> MLPQDDMTDEMKSLASRLEDTTQA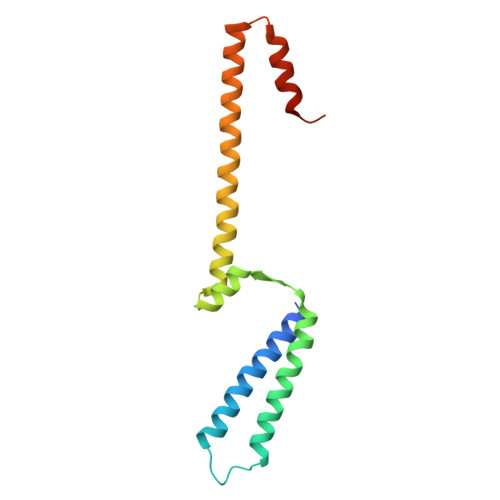FYDLALIVYNLEDTTPSDAIPESLDTLIRDLKSLPDISRKVNNLIPQDVLEYIEQGRNPDVYARQFSELVQKDNQYVNGKLYAIEGFQKAFAEEIKQAYPEVSSVVDKILNEGKVESTVS> MGHHHHHHMTTDDLLTRYRANPAMMKNLKLSDIRGALLKFAKDQVGSRFIQQELASSKDRFEKDSIFDEVV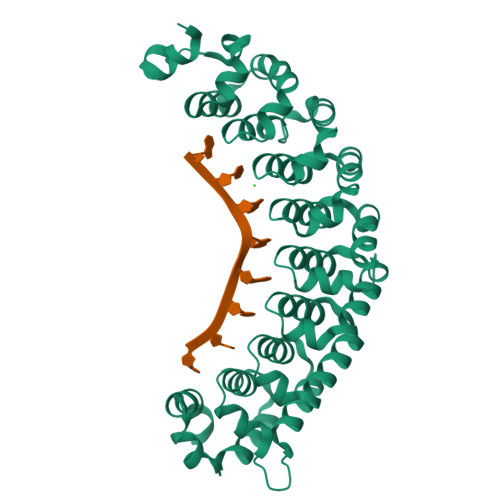SNADELVDDIFGNYVVQKFFEYGEERHWARLVDAIIDRVPEYAFQMYACRVLQKALEKINEPLQIKILSQIRHVIHRCMKDQNGNHVVQKAIEKVSPQYVQFIVDTLLESSNTIYEMSVDPYGCRVVQRCLEHCSPSQTKPVIGQIHKRFDEIANNQYGNYVVQHVIEHGSEEDRMVIVTRVSNNLFEFATHKYSSNVIEKCLEQGAVYHKSMIVGAACHHQEGSVPIVVQMMKDQYANYVVQKMFDQVTSEQRRELILTVRPHIPVLRQFPHGKHILAKLEKYFQKPA> KKNTAASLQQWKVGDKCSAIWSEDGCIYPATIASIDFKRETCVVVYTGYGNREEQNLSDLLSPI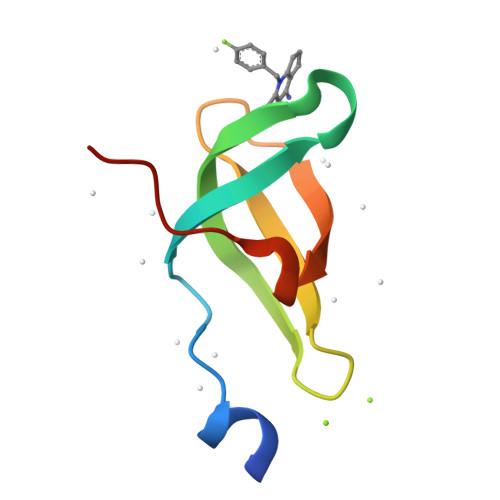CE> A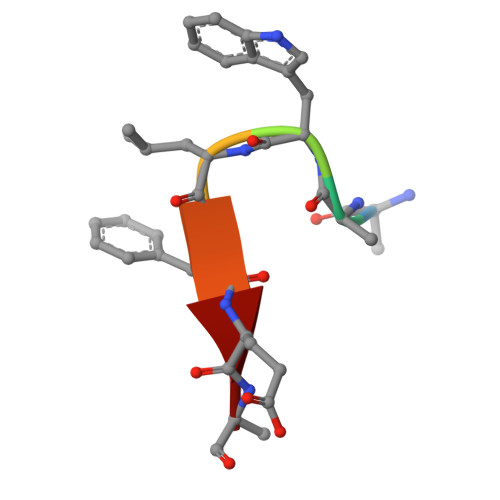AWLFEA>[2x]MSLAHKFDPSKIKKLDDPSRLELFDPEKVLKEFGLKEGMTVLDVGTGAGFYLPYLSKMVGEKGKVY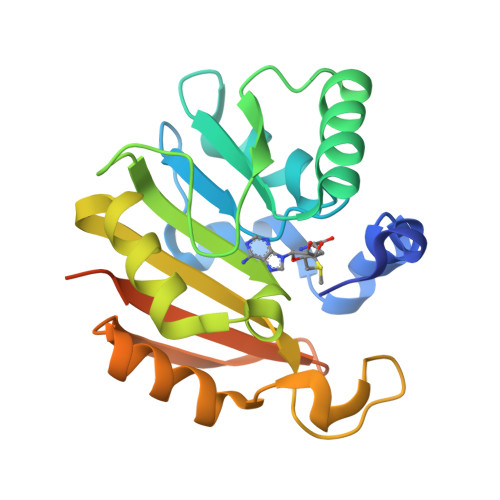AIDVQEEMVNYAWEKVNKLGLKNVEVLKSEENKIPLPDNTVDFIFMAFTFHELSEPLKFLEELKRVAKPFAYLAIIDWKKEERDKGPPPEEVYSEWEVGLILEDAGIRVGRVVEVGKYCFGVYAMIVKQEEENPLMNVPFKIPPGEGHHHHHH>[2x]APTENSTGVQDCYRGDGQSYRGTLSTTITGRTCQSWSSMTPHWHRRIPLYYPNAGLTRNYCRNPDAEIRPWCYTMDPSVRWEYCNLTRCPVTES

Lipoprotein(a) (Lp(a)), an independent, causal cardiovascular risk factor, is a lipoprotein particle that is formed by the interaction of a low-density lipoprotein (LDL) particle and apolipoprotein(a) (apo(a)). Lp(a) is a lipoprotein particle that is formed by a two-step process involving interactions between a LDL particle and another protein, apo(a). The goal of our research was to develop a potent and selective orally delivered small-molecule therapeutic to inhibit the formation of Lp(a) by blocking the first interaction between apo(a) and apoB to reduce the circulating levels of Lp(a). In summary, we report the discovery and optimization of potent and selective small-molecule inhibitors of Lp(a) formation by exploiting the repeated KIV domain structure of apo(a) through compound multivalency.

Crystal structure analysis showed that LSN3353871 interacts with the KIV8 amino acid residues Glu56, Asp54, Tyr62 and Arg69, illustrating the specificity and binding modality of the molecule. The structural data with LSN3353871 revealed a molecular interaction between a key motif made up of an aspartic acid (D) residue, any amino acid (x) and a glutamic acid residue (E) (DxE motif) in KIV8, so we focused on the presence of these motifs in plasminogen. Notably, in apo(a), each KIV repeat from KIV5 through to KIV8 contains the DxE motif. In an in vitro Lp(a) assembly assay, LSN3353871 disrupted the formation of Lp(a) with a half-maximal inhibitory concentration (IC50) of 1.69 µM (n = 43). Oral administration of LSN3353871 to mice expressing human Lp(a) resulted in dose-dependent increases in the circulating levels of LSN3353871 and dose-dependent decreases of up to 78% in the levels of Lp(a), with a median effective dose (ED50) of 14 mg kg−1 twice daily (BID) within five days of dosing. In cynomolgus monkeys, administration of LSN3353871 (20 mg kg−1 BID for two weeks) resulted in a decrease of up to 40% in the levels of Lp(a). The difference in the magnitude of effect between these two models could be explained by differences in the expression levels and metabolism of Lp(a), because the mouse genome does not inherently contain the LPA gene. These data provide a proof of concept that a small molecule that binds to the lysine-binding domains of apo(a) can inhibit the formation of Lp(a) in vivo.>[12x]MKLTPKELDKLMLHYAGELARKRKEKGIKLNYVEAVALISAHIMEEARAGKKTAAELMQEGRTLLKPDDVMDGVASMIHEVGIEAMFPDGTKLVTVHTPIEANGKLVPGELFLKNEDITINEGKKAVSVKVKNVGDRPVQIGSHFHFFEVNRCLDFDREKTFGKRLDIASGTAVRFEPGEEKSVELIDIGGNRRIFGFNALVDRQADNESKKIALHRAKERGFHGTKSDDNYVKTIKE;>MKKISRKEYVSMYGPTTGDKVRLGDTDLIAEVEHDYTIYGEELKFGGGKTLREGMSQSNNPSKEELDLIITNALIVDYTGIYKADIGIKDGKIAGIGKGGNKDMQDGVKNNLSVGPATEALAGEGLIVTAGGIDTHIHFISPQQIPTAFASGVTTMIGGGTGPADGTNATTITPGRRNLKWMLRAAEEYSMNLGFLAKGNTSNDASLADQIEAGAIGFKIHEDWGTTPSAINHALDVADKYDVQVA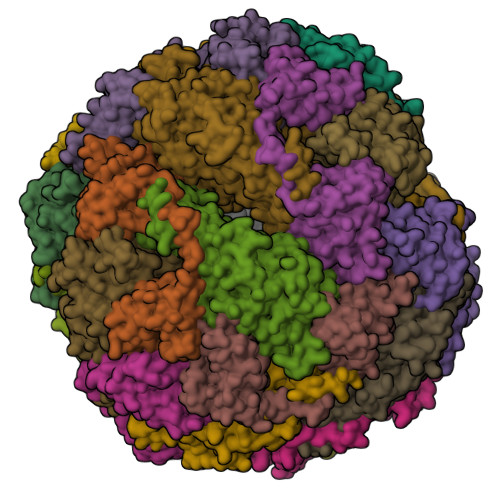IHTDTLNEAGCVEDTMAAIAGRTMHTFHTEGAGGGHAPDIIKVAGEHNILPASTNPTIPFTVNTEAEHMDMLMVCHHLDKSIKEDVQFADSRIRPQTIAAEDTLHDMGIFSITSSDSQAMGRVGEVITRTWQTADKNKKEFGRLKEEKGDNDNFRIKRYLSKYTINPAIAHGISEYVGSVEVGKVADLVLWSPAFFGVKPNMIIKGGFIALSQMGDANASIPTPQPVYYREMFAHHGKAKYDANITFVSQAAYDKGIKEELGLERQVLPVKNCRNITKKDMQFNDTTAHIEVNPETYHVFVDGKEVTSKPANKVSLAQLFSIF[12x]>MDYKDDDDKGSSTSLYKKAGSETLYIQGQDEYYMARALKLAQRGRFTTHPNPNVGCVIVKDGEIVGEGYHQRAGEPHAEVHALRMAGEKAKGATAYVTLEPCSHHGRTPPCCDALIAAGVARVVASMQDPNPQVAGRGLYRLQQAGIDVSHGLMMSEAEQLNKGFLKRMRTGFPYIQLKLGASLDGRTAMASGESQWITSPQARRDVQLLRAQSHAILTSSATVLADDPALTVRWSELDEQTQALYPQQNLRQPIRIVIDSQNRVTPVHRIVQQPGETWFARTQEDSREWPETVRTLLIPEHKGHLDLVVLMMQLGKQQINSIWVEAGPTLAGALLQAGLVDELIVYIAPKLLGSDARGLCTLPGLEKLADAPQFKFKEIRHVG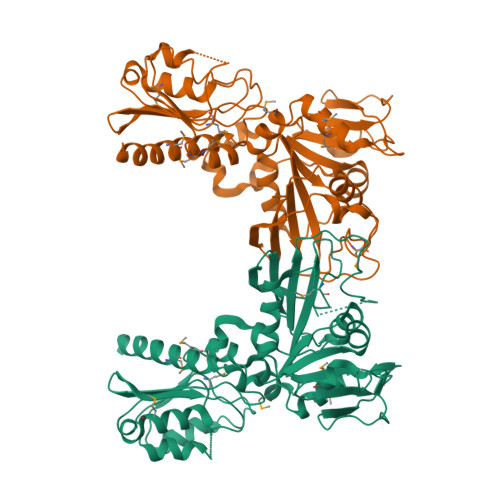PDVCLHLVGASTHHHHHH[2x]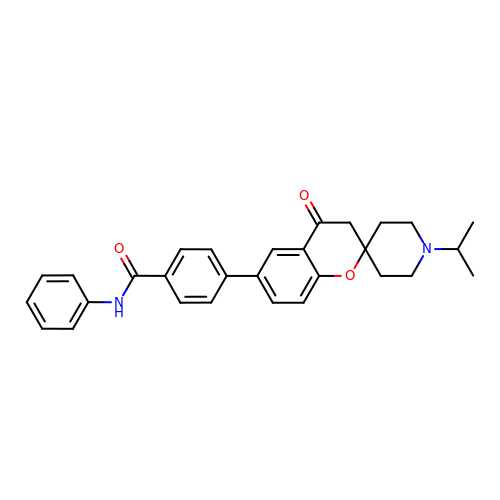4-(4-oxidanylidene-1'-propan-2-yl-spiro[3~{H}-chromene-2,4'-piperidine]-6-yl)-~{N}-phenyl-benzamide | C29 H30 N2 O3 | XQDWUPXCNFCIBY-UHFFFAOYSA-N>[24x]MANPTLFVSYDQNGKKLSFANWISVLSPQDTPFVSMTGKESINQTIFSWQTDALASVDGNNAHVEGSRAEDGEMKPTVIKSNVTQILRKVVRVSDTANTTANYGRGRELMYQLEKKGKEIKRDLEKILLSGQARTDVLADQYLTNSAADPAVAGLNDTHAARKTGAFQFLCAHGGLAGGVVDKTKNGPADPDTGAVTVKVAQNASNPTTNIGFDEADIFDMTLQLYTAGSEADIIMINPAHAKIFAGLQENTQGSRKRIFENTKQFIYEVNSITDPLGQSYKIIVNRWMPTDAVYFFRSADWTQMVLRAPKRTELAKDGSYEKWMIEMEVGLRHRNPYASGVLFTAAGKAAA

Escherichia coli phage SU10 belongs to the genus Kuravirus from the class Caudoviricetes of phages with short non-contractile tails. Here we show that the virion of SU10 has a prolate head, containing genome and ejection proteins, and a tail, which is formed of portal, adaptor, nozzle, and tail needle proteins and decorated with long and short fibers. In contrast to other short-tailed phages, the tails of Kuraviruses elongate upon cell attachment. After binding to the host, SU10 tail, nozzle proteins, and short fibers re-arrange to form a nozzle that extends the tail.

The central tubular part of the capsid is built from 90 hexamers arranged in nine layers of a ten-entry helix. The hexamers in the caps are more bent (H4, H5; 149-150°), whereas those that form the tubular part of the capsid are relatively flat (H1, H2L, H2R, H3; 154–164°). All hexamer-hexamer and hexamer-pentamer interfaces in the caps are arched (145°), however, the hexamers that form the tubular part of the capsid are connected by two types of interfaces, arched (145°) and more planar (160°). The arched interfaces enable the formation of rings of hexamers, whereas the more planar ones mediate interactions between the rings. In hexamers, the annular loop protrudes away from the axial domain. The six annular loops from subunits forming one hexamer form a ring around its quasi-sixfold axis. Nine shells of density can be distinguished inside the tubular part of the head, whereas only four shells are resolved underneath the capsid caps. In both five-fold symmetric and asymmetric reconstructions of the SU10 head, the DNA strands in the two outermost layers are organized as ten-entry helices.> MSRKKMGLLVMAYGTPYKEEDIERYYTHIRRGRKPEPEMLQDLKDRYEAIGGISPLAQITEQQAHNLEQHLNEIQDEITFKAYIGLKHIEPFIEDAVAEMHKDGITEAVSIVLAPHFSTFSVQSYNKRAKEEAEKLGGLTITSVESWYDEPKFVTYWVDRVKETYASMPEDERENAMLIVSAHSLPEKIKEFGDPYPDQLHESAKLIAEGAGVSEYAVGWQSEGNTPDPWLGPDVQDLTRDLFEQKGYQAFVYVPVGFVADHLEVLYD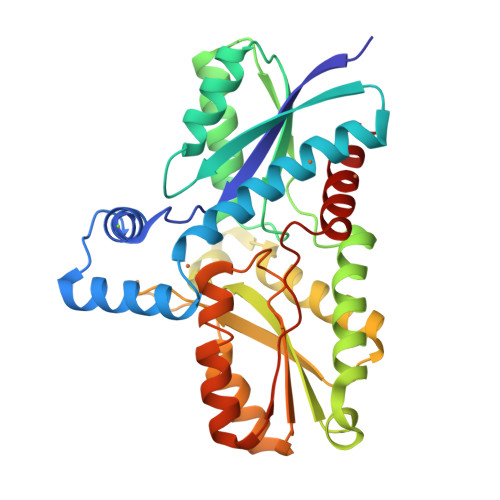NDYECKVVTDDIGASYYRPEMPNAKPEFIDALATVVLKKLGR> ATQSPGDSRRLSIQRAIQSLVHAAQCRNANCSLPSCQKMKRVVQHTKGCKRKTNGGCPI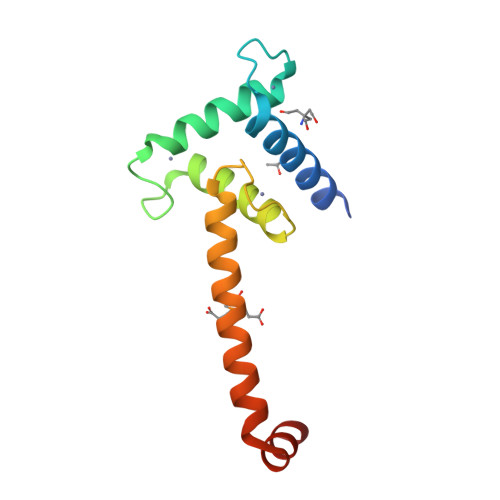CKQLIALAAYHAKHCQENKCPVPFCLNIKQKLRQQQLEASIDLSAYIESGEEQLLSDLFAVK Chondroitin sulfate A is a linear, sulfated carbohydrate linked to periodontal disease as the principal species of glycosaminoglycan appended on the surface of cortical bone of teeth and in supporting dental ligaments. Through genomic comparisons with B. thetaiotaomicron, a new PUL-like operon (Bfo2285-Bfo2295, and Bfo3043) was identified in T. forsythia and the crystal structure of two proteins from this PUL-like operon, Bfo2290 and Bfo2294, were reported using X-ray crystallography. Here we define a pathway for the degradation of CSA by T. forsythia based on the discovery of a PUL-like gene cluster found using bioinformatics analysis, functionally characterize three proteins (Bfo2285, Bfo2290, Bfo2291, and Bfo2294) from this PUL-like gene cluster and report the crystal structure of an exo-N-acetylgalactosamine (Bfo2290) and for a 2-keto-3-deoxy-6-phosphogluconate (KDPG) and 2-keto-4-hydroxyglutarate (KHP) to D-glyceraldehyde-3-phosphate aldolase (Bfo2294). As CSA is the primary GAG in alveolar bone, this likely serves as a mechanism by which T. Forsythia compromises periodontal tissues contributing to bone loss in periodontal disease in conjunction with host osteoclastic activity.

The structure was solved to a resolution of 2.85 Å in the space group of P212121 and iteratively built and refined to a corresponding Rwork of 0.230 and an Rfree of 0.276. The refined model contained 3 protein molecules in the asymmetric unit arrange as a trimer with C3 symmetry. The model contained an α/β topology shown using a topological diagram of the polypeptide fold with 13 β-strands (β1-β13), and 16 α-helices (α1-α16). Two distinct domains were observed with the larger one containing a 9-strand parallel β sheet (N-terminal domain) with the exception of β4 and β8 which were anti-parallel. The smaller second domain (C-terminal domain) contained a beta sheet consisting of 4 anti-parallel beta strands (β10-β13) and a long alpha helical region (α16) running orthogonal to the β strands but in the same plane as a solvent exposed structure. Topologically Bfo2290 was very similar to BT3349 from B. thetaiotaomicron. The superimposed structures had a final alignment root mean squared deviation (RMSD) of 1.105 Å, structural distance measure (SDM) of 11.021 with a cutoff of 10, and a Q-score of 0.797. When Bfo2290 and BT3349 were superimposed, it was found that many of the residues found in the binding pocket were positively charged residues or polar nitrogen containing residues with a positive dipole facing the substrate modeled in the BT3349 co-crystal structure. Although current experimental evidence supports an exolytic catalytic mechanism, or a high preference for ΔDi-4S, the only major structural difference noted between Bfo2290 and BT3349 (an endolytic sulfatase), is the absence of a bound calcium cation metal cofactor.

>MKASKLSCLGLIGVIPACIHAQEHRADDTLRPNIIYIFPDQMRNSAMGFWNDPAFASHLQGKADPVETPNLNRFARESVVFSSAMSNCPLSSPHRASLLTGMYPHRSGVPLNVNSRRPFSTLRNDATTVSDVFSRNGYDCAYIGKYHLDTPTPNDPENPGNYVENRDLVWDAYTPPERRHGFNFWYSYGTFDVHKHPHYWDTDGKRHDINQWSPSHETDMAISYLKNEFGRRDVSKPFFLMISMNPPHHPYNSFNDCMEEDYTHYKDRTLSELLVRHNADTTMEKSSSAAYYFAQITGVDREFGRLLEALDELGLSKNTMVVFSSDHGETMCSHGLQDAKNSPYIESMNVPFLIRYPQRLKPKVVDYLLSSPDIMPTLLGLSNLGQHIPHEVQGTDFSKALFSNQPDKPLPDAALYIRNMDGRQDQDGKVRTYVPVARGIKTHRYTLSLTVDKENKQLKEILLFDDLDDPYQMNNIDWNTRPQLKRQLLIQLGQLLKKYDDPWYKDGILKDLIMYE[3x]>HHHHHHMALQLAAHSDARSGPVGSNGGQFWSFRPVRPLNKIVLSFSGSPDQTLNLISITFSSNPTDIITVGGVGPEPLTYTETVNIDGDIIEISGMIANYKGYNVIRSIKFTTNKKEYGPYGANAGTPFNIKIPDGNKIVGFFGNSGWYVDAIGAYYTAK[4x]

Structural and functional analysis identified IPO as a member of the JRL family but with a different tetrameric association. The monomeric IPO from residues 1 to 154 shows a typical β-prism fold found in the JRL family, with 12 β-sheets (β3-β14) and 2 additional short, extended, N-terminal β-strands (β1-β2). Four IPO protomers form a compact tetrameric association by swapping their extended N termini from residues 1 to 10. Thus, the wound-inducible protein IPO from sweet potato has versatile carbohydrate binding properties and might play a role in plant defense.

The crystal of IPO–Me-Glc was determined to be a monoclinic space group P21. The Matthews coefficient and solvent content was 2.26 Å3/Da and 45.5% for 4 molecules. In addition, the resolved structure of IPO–Me-Glc formed a tetrameric association. We analyzed the tetrameric association of IPO–Me-Glc. The 2 extended N termini from monomer A in blue and monomer B in purple swap with each other. Consequently, a larger buried interface between monomers A and B is 1,522 Å2. In the chain A of IPO–Me-Glc, 9 hydrogen bonds are formed by the residues Gly21, Tyr97, Gly141, Trp142, Tyr143 and Asp145 of IPO and the atoms O1, O3, O4, O5, and O6 of Me-Glc. The atom C7 of Me-Glc is involved in the methyl carbon (Me)…π interaction with Trp142 of IPO. In chains B to D, the Cd2+ atom forms 5 coordinates by the O atom of the carbonyl group of Asn19, OG atom of Ser18, and 3 water molecules. One of the 3 water molecules forms a hydrogen bond with Asp145.We found a previously uncharacterized protein classified as a glycosyltransferase encoded in the Actinobacillus minor NM305 genome and named the gene product A. minor glucoside-glucosyltransferase (AmGGT). AmGGT exhibited processive glycosyltransferase activity when UDP-Glc was used as the donor substrate and, unexpectedly, showed different acceptor substrate specificity from that of the homologous Agt proteins of other Actinobacillus species. While the homologous proteins transfer glucose residues to the nonreducing end of oligosaccharide chains linked to peptides, AmGGT cannot use glycopeptides as acceptors and requires the nonreducing end of oligosaccharides. The AmGGT protein consists of two lobe domains, which are typically found in the GT-B fold proteins.

The crystal structure of the AmGGT protein was determined to the resolution of 1.85 Å. Although the AmGGT protein was mixed with isomaltose (as an acceptor), no density corresponding to the isomaltose molecule was present in the electron density map, presumably due to the weak affinity of isomaltose for the AmGGT protein. A substrate-binding groove is formed at the interface between the two lobe domains. Although the asymmetric unit contained one molecule of the AmGGT protein, the gel-filtration chromatography suggested that the AmGGT protein exists as a homodimer in solution. A dimeric structure was generated according to the 2-fold rotational crystal lattice symmetry. No protein degradation was observed with the E135A-S185A mutant protein. In sum, the AmGGT protein is a homodimer with 2-fold rotational symmetry in solution. In contrast, at 37 °C, the catalytic activity of the WT protein increased, but that of the E135A-S185A mutant protein decreased. These results suggest that the homodimeric structure of the AmGGT protein contributes to its thermal stability under physiological temperature conditions in the porcine host. In the AmGGT structure, the side chain of Tyr16 protrudes into the substrate-binding groove, narrowing the acceptor-binding site. This bulged structure likely prevents the binding of glycopeptide substrates, such as the Glc1-peptide, to the acceptor-binding site.

> GPSNITFYFPFGHVPTYGGDFVNLEHIRALNKHGFSAKVILMKNQIPIVIESFPKDIPVVFYKPGMELNAQDVFVLSEGVRIMYSGLAQTQAFRVIVHNQNPFYTHTGMDSAHDINRYRITKIITPSHYTVKKLEEMGITKPMAVISPYIPEYFKPAEKSNEEIRITYSRRKREEESKILLFYLRSLYRGKKALHIRNLTNYKREEVAEEMSKAHIYASFAERESLGLMALEAMASGCHVVGFSGFTDFENQDVFNEENGDWVKEGEYKKFAEKLIEAIEQIENNTPSPKIENGLALVNSRFRQDRFEQEVVRVYQDILDNLPPLEGFNESDKVVLDFWHFD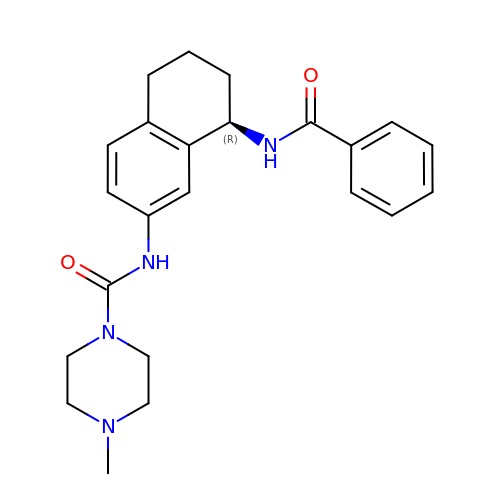N-[(8R)-8-(benzoylamino)-5,6,7,8-tetrahydronaphthalen-2-yl]-4-methylpiperazine-1-carboxamide | C23 H28 N4 O2 | QTWWLOSRVGQGNN-OAQYLSRUSA-N>[2x]MAQSMYPNEPIVVVGSGCRFPGDANTPSKLWELLQHPRDVQSRIPKERFDVDTFYHPDGKHHGRTNAPYAYVLQDDLGAFDAAFFNIQAGEAESMDPQHRLLLETVYEAVTNAGMRIQDLQGTSTAVYVGVMTHDYETVSTRDLESIPTYSATGVAVSVASNRISYFFDWHGPSMTIDTACSSSLVAVHLAVQQLRTGQSSMAIAAGANLILGPMTFVLESKLSMLSPSGRSRMWDAGADGYARGEAVCSVVLKTLSQALRDGDTIECVIRETGVNQDGRTTGITMPNHSAQEALIKATYAQAGLDITKAEDRCQFFEAHGTGTPAGDPQEAEAIATAFFGHEQVARSDGNERAPLFVGSAKTVVGHTEGTAGLAGLMKASFAVRHGVIPPNLLFDKISPRVAPFYKNLRIPTEATQWPALPPGQPRRASVNSFGFGGTNAHAIIEEYMEPEQNQLRVSNNEDCPPMTGVLSLPLVLSAKSQRSLKIMMEEMLQFLQSHPEIHLHDLTWSLLRKRSVLPFRRAIVGHSHETIRRALEDAIEDGIVSSDFTTEVRGQPSVLGIFTGQGAQWPGMLKNLIEASPYVRNIVRELDDSLQSLPEKYRPSWTLLDQFMLEGEASNVQYATFSQPLCCAVQIVLVRLLEAARIRFTAVVGHSSGEIACAFAAGLISASLAIRIAYLRGVVSAGGARGTPGAMLAAGMSFEEAQEICELDAFEGRICVAASNSPDSVTFSGDANAIDHLKGMLEDESTFARLLKVDTAYHSHHMLPCADPYMQALEECGCAVADAGSPAGSVPWYSSVDAENRQMAARDVTAKYWKDNLVSPVLFSHAVQRAVVTHKALDIGIEVGCHPALKSPCVATIKDVLSGVDLAYTGCLERGKNDLDSFSRALAYLWERFGASSFDADEFMRAVAPDRPCMSVSKLLPAYPWDRSRRYWVESRATRHHLRGPKPHLLLGKLSEYSTPLSFQWLNFVRPRDIEWLDGHALQGQTVFPAAGYIVMAMEAALMIAGTHAKQVKLLEILDMSIDKAVIFDDEDSLVELNLTADVSRNAGEAGSMTISFKIDSCLSKEGNLSLSAKGQLALTIEDVNPRTTSASDQHHLPPPEEEHPHMNRVNINAFYHELGLMGYNYSKDFRRLHNMQRADLRASGTLDFIPLMDEGNGCPLLLHPASLDVAFQTVIGAYSSPGDRRLRCLYVPTHVDRITLVPSLCLATAESGCEKVAFNTINTYDKGDYLSGDIVVFDAEQTTLFQVENITFKPFSPPDASTDHAMFARWSWGPLTPDSLLDNPEYWATAQDKEAIPIIERIVYFYIRSFLSQLTLEERQQAAFHLQKQIEWLEQVLASAKEGRHLWYDPGWENDTEAQIEHLCTANSYHPHVRLVQRVGQHLLPTVRSNGNPFDLLDHDGLLTEFYTNTLSFGPALHYARELVAQIAHRYQSMDILEIGAGTGGATKYVLATPQLGFNSYTYTDISTGFFEQAREQFAPFEDRMVFEPLDIRRSPAEQGFEPHAYDLIIASNVLHATPDLEKTMAHARSLLKPGGQMVILEITHKEHTRLGFIFGLFADWWAGVDDGRCTEPFVSFDRWDAILKRVGFSGVDSRTTDRDANLFPTSVFSTHAIDATVEYLDAPLASSGTVKDSYPPLVVVGGQTPQSQRLLNDIKAIMPPRPLQTYKRLVDLLDAEELPMKSTFVMLTELDEELFAGLTEETFEATKLLLTYASNTVWLTENAWVQHPHQASTIGMLRSIRREHPDLGVHVLDVDAVETFDATFLVEQVLRLEEHTDELASSTTWTQEPEVSWCKGRPWIPRLKRDLARNNRMNSSRRPIYEMIDSSRAPVALQTARDSSSYFLESAETWFVPESVQQMETKTIYVHFSCPHALRVQALGFFYLVQGHVQEGNREVPVVALAERNASIVHVRPDYIYTEADNNLSEGGGSLMVTVLAAAVLAETVISTAKCLGVTDSILVLNPPSICGQMLLHAGEEIGLQVHLATTSGNRSSVSAGDAKSWLTLHARDTDWHLRRVLPRGVQALVDLSADQSCEGLTQRMMKVLMPGCAHYRAADLFTDTVSTELHSGSRHQASLPAAYWEHVVSLARQGLPSVSEGWEVMPCTQFAAHADKTRPDLSTVISWPRESDEATLPTRVRSIDAETLFAADKTYLLVGLTGDLGRSLGRWMVQHGACHIVLTSRNPQVNPKWLAHVEELGGRVTVLSMDVTSQNSVEAGLAKLKDLHLPPVGGIAFGPLVLQDVMLNNMELPMMEMVLNPKVEGVRILHEKFSDPTSSNPLDFFVMFSSIVAVMGNPGQANYSAANCYLQALAQQRVASGLAASTIDIGAVYGVGFVTRAELEEDFNAIRFMFDSVEEHELHTLFAEAVVAGRRAVHQQEQQRKFATVLDMADLELTTGIPPLDPALKDRITFFDDPRIGNLKIPEYRGAKAGEGAAGSKGSVKEQLLQATNLDQVRQIVIDGLSAKLQVTLQIPDGESVHPTIPLIDQGVDSLGAVTVGTWFSKQLYLDLPLLKVLGGASITDLANEAAARLPPSSIPLVAATDGGAESTDNTSENEVSGREDTDLSAAATITEPSSADEDDTEPGDEDVPRSHHPLSLGQEYSWRIQQGAEDPTVFNNTIGMFMKGSIDLKRLYKALRAVLRRHEIFRTGFANVDENGMAQLVFGQTKNKVQTIQVSDRAGAEEGYRQLVQTRYNPAAGDTLRLVDFFWGQDDHLLVVAYHRLVGDGSTTENIFVEAGQLYDGTSLSPHVPQFADLAARQRAMLEDGRMEEDLAYWKKMHYRPSSIPVLPLMRPLVGNSSRSDTPNFQHCGPWQQHEAVARLDPMVAFRIKERSRKHKATPMQFYLAAYQVLLARLTDSTDLTVGLADTNRATVDEMAAMGFFANLLPLRFRDFRPHITFGEHLIATRDLVREALQHARVPYGVLLDQLGLEVPVPTSNQPAPLFQAVFDYKQGQAESGTIGGAKITEVIATRERTPYDVVLEMSDDPTKDPLLTAKLQSSRYEAHHPQAFLESYMSLLSMFSMNPALKLAHVHHHHHH;>MGDQPFIPPPQQTALTVNDHDEVTVWNAAPCPMLPRDQVYVRVEAVAINPSDTKMRGQFATPWAFLGTDYAGTVVAVGSDVTHIQVGDRVYGAQNEMCPRTPDQGAFSQYTVTRGRVWAKIPKGLSFEQAAALPAGISTAGLAMKLLGLPLPSPSADQPPTHSKPVYVLVYGGSTATATVTMQMLRLSGYIPIATCSPHNFDLAKSRGAEEVFDYRAPNLAQTIRTYTKNNLRYALDCITNVESTTFCFAAIGRAGGHYVSLNPFPEHAATRKMVTTDWTLGPTIFGEGSTWPAPYGRPGSEEERQFGEDLWRIAGQLVEDGRLVHHPLRVVQGGFDHIKQGMELVRKGELSGEKLVVRLEGPLEHHHHHH[2x]

The first isolable intermediate of the lovastatin biosynthetic pathway, dihydromonacolin L (DML), is constructed by the highly reducing iterative polyketide synthase (HR-iPKS) LovB, which partners with LovC, an enoyl reductase that acts in trans. In LovB, the β-ketoacyl synthase (KS), malonyl-acetyl transferase (MAT), dehydratase (DH), methyltransferase (CMeT), acyl carrier protein (ACP), and ketoreductase (KR) domains are active, except for the enoyl reductase (ER) domain. LovB terminates with a condensation (CON) domain commonly found in nonribosomal peptide synthetases. In DML biosynthesis by LovB, the initiation and elongation of the intermediate chain are carried out by the KS, MAT, and ACP domains. ß-Ketoacyl modification cycles are also repeated, but the tailoring domain usage during each iteration is highly programmed and permutative.

The structure of LovB adopts an X-shaped dimer architecture, and the LovBC complex reveals the position of LovC which binds to the MAT domain of LovB, forming two complete L-shaped catalytic chambers. The LovBC complex adopts an X shape in the front view with two wings. Starting from the lower region, the KS and MAT domains are connected by the linker domain (LD), with the separate ER (LovC) domain interacting with the MAT domain. LovB alone is ~176 Å wide, while the LovBC complex is ~294 Å wide. The adoption of a pseudo-twofold face-to-face symmetry of LovB, in connection with LovC, creates two L-shaped catalytic chambers. The chamber is chimeric, with the KS, and MAT domains coming from one chain, and the DH, CMeT, ψKR, ψER, and KR domains from another. The LovB–C interface is approximately 522 Å2, which is mainly contributed by several residues in the loop region of LovC and α helices of the MAT domain. At the same time, the MAT domain Mut1 abolished interaction with LovC. These observations suggest that the loop within LovC and the helix of MAT domain of LovB are essential for the formation of the LovBC complex. The significance of LovB–LovC binding for the integrity of the catalytic chamber was analyzed by an in vitro reaction assay catalyzed by LovB–LovC and LovG. Figure 4e shows that the interface mutation abolished the synthesis of DML acid, in spite of the full catalytic competence of the mutant. We conclude that the formation of the LovBC complex is essential for the integrity of the catalytic chamber to the complete total synthesis of DML acid.> QIRSLCELYGYWSGNGYELLNNLWGKDTATSGWQCTYLDGTNNGGIQWSTAWEWQGAPDNVK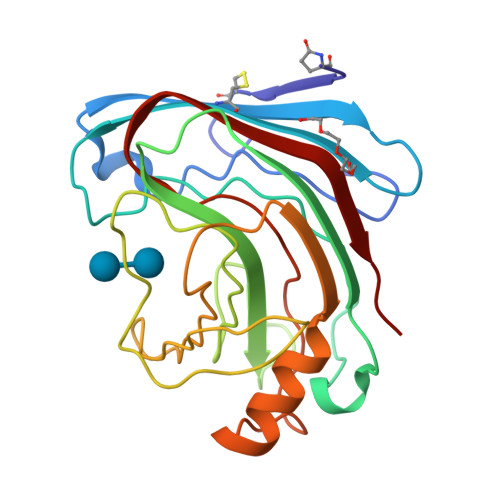SYPYVGKQIQRGRKISDINSMRTSVSWTYDRTDIRANVAYDVFTARDPDHPNWGGDYELMIWLARYGGIYPIGTFHSQVNLAGRTWDLWTGYNGNMRVYSFLPPSGDIRDFSCDIKDFFNYLERNHGYPAREQNLIVYQVGTECFTGGPARFTCRDFRADLW>EGVECDFSPLLSGTPPQVYNFKRLVFTNCNYNLTKLLSLFSVNDFTCSQISPAAIASNCYSSLILDYFSYPLSMKSDLSVSSAGPISQFNYKQSFSNPTCLILATVPHNLTTITKPLKYSYINKCSRLLSDDRTEVP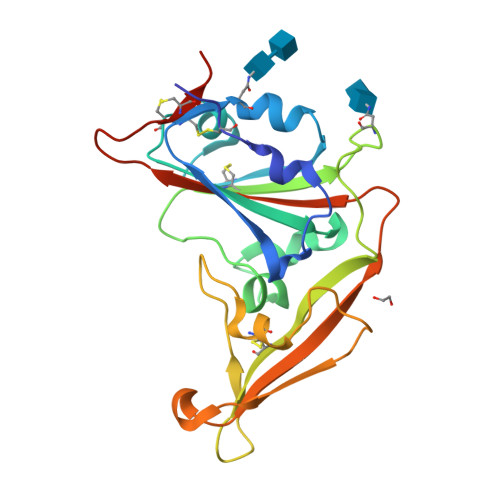QLVNANQYSPCVSIVPSTVWEDGDYYRKQLSPLEGGGWLVASGSTVAMTEQLQMGFGITVQYGTDTNSVCPKLHHHHHH[2x]>MAADNPYQRGPDPTNASIEAATGPFAVGTQPIVGASGFGGGQIYYPTDTSQTYGAVVIVPGFISVWAQLNWLGPRLASQGFVVIGIETSVITDLPDPRGDQALAALDWATTRSPVASRIDRTRLAAAGWSMGGGGLRRAALQRPSLKAIVGMAPWNGERNWSAVTVPTLFFGGSSDAVASPNDHAKPFYNSITRAEKDYIELRNADHFFPTSANTTMAKYFISWLKRWVDNDTRYTQFLCPGPSTGLFAPVSASMNTCPFLEHHHHHH[2x]

In the present study, we report a PET hydrolase from Cryptosporangium aurantiacum (CaPETase) that exhibits remarkable PET degradation activity at ambient temperatures and high thermostability. CaPETase shows an α/β hydrolase fold and a nine-stranded β-sheet at the center surrounded by six α-helices and two 310-helices. Formation of one conserved disulfide bond (DS, C279/C297) and lack of an extended loop in the substrate binding site of CaPETase suggest that the enzyme originated from an ancestor of TfCut2 and LCC rather than IsPETase.

To provide a structural basis for high PET hydrolytic activity of CaPETase, we determined its crystal structure at a resolution of 1.36 Å. Interestingly, CaPETase exhibits a somewhat different backbone structure at the active site compared with other PET hydrolases. Interestingly, CaPETase also showed significant differences in the backbone torsion angles at the five connecting loops (β3–α1, β4–α2, β6–β7, β7–α4, and β8–α5) that form an active site, whereas comparisons of the corresponding loops between the other three PET hydrolases exhibited less differences, suggesting that CaPETase has a unique active site conformation. Near the β3–α1 loop, distinct residues positioned in the β4–α2 loop and a W105–L108–G124 network force, which form a unique side-chain internal network, appear to influence the conformation of the β3–α1 loop. A unique A192–G212–F248 network is formed under the β8–α5 loop, where catalytic H246 is located. Therefore, the positioning of a bulky F248 might cause significant torsional differences in the β8–α5 loop and β7–α4 loop of CaPETase. Finally, an R176–W200–F209 network appears to trigger conformational differences in the α3-helix and β6–β7 loop. In addition to the unique backbone conformation at the active site, residues forming the substrate binding cleft of CaPETase showed significant differences compared with other thermophilic PET hydrolases. CaPETase also contains a unique I102 residue in the β3–α1 loop showing the largest torsion differences, whereas other PET hydrolases contain a highly conserved threonine residue at the corresponding position, which probably enables CaPETase to form a relatively wider substrate binding cleft. Taken together, we suggest that along with unique backbone torsion angles, the positioning of distinct residues at the substrate binding site enable CaPETase to form an optimal substrate binding site for high PET hydrolytic activity.>MAVLHINALDQLTALLSTEKVIVIDFFATWCGPSRSISPYFEELAGQYNNIKFVKVDVDQAEEICVNYKVRSMPTFVLVKDGI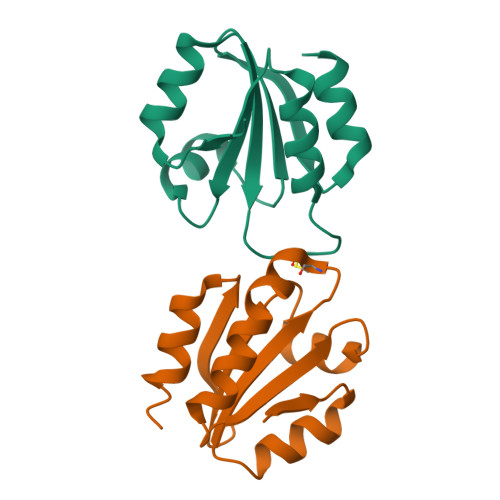EQKRFSGADRNALKQMVETAHHHHHH[2x]>[6x]SPDPNW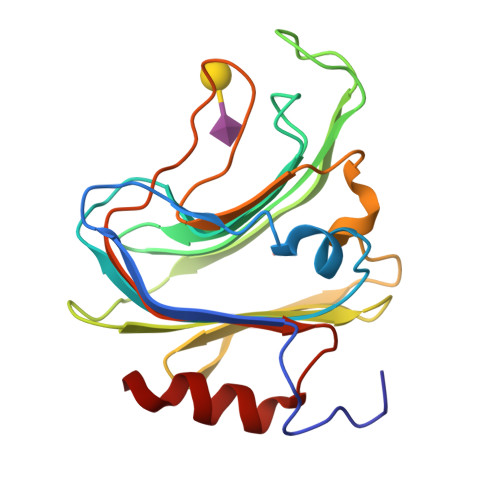ELLSSLGEYKDINLESSNASNITYDLEKYKNLDEGTIVVRFNSKDSKIQSLLGISNSKTKNGYFNFYVTNSRVGFELRNQKNEGNTQNGTENLVHMYKDVALNDGDNTVALKIEKNKGYKLFLNGKMIKEVKDTNTKFLNNIENLDSAFIGKTNRYGQSNEYNFKGNIGFMNIYNEPLGDDYLLSKTGETK>[2x]FNEPLNIVSHLNDDWFLFGDARSDCTYVENNGHPKLDWLDLDPKLCNSGRISAKSGNSLFRSFHFIDFYNYSGEGDQVIFYEGVNFSPSHGFKCLAYGDNKRWMGNKARFYARVYEKMAQYRSLSFVNVSYAYGGNAKPTSICKDKTLTLNNPTFISKESNYVDYYYESEANFTLQGCDEFIVP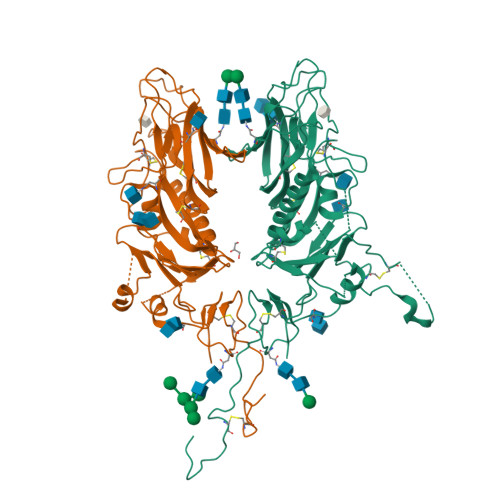LCVFNGHSKGSSSDPANKYYTDSQSYYNMDTGVLYGFNSTLDVGNTVQNPGLDLTCRYLALTPGNYKAVSLEYLLSLPSKAICLRKPKSFMPVQVVDSRWNSTRQSDNMTAVACQLPYCFFRNTSADYSGGTHDVHHGDFHFRQLLSGLLYNVSCIAQQGAFVYNNVSSSWPAYGYGHCPTAANIGYMAPVCIYDSDPLVPR>[4x]MTQQITLIKDKILSDNYFTLHNITYDLTRKDGEVIRHKREVYDRGNGATILLYNTKKKTVVLIRQFRVATWVNGNESGQLIE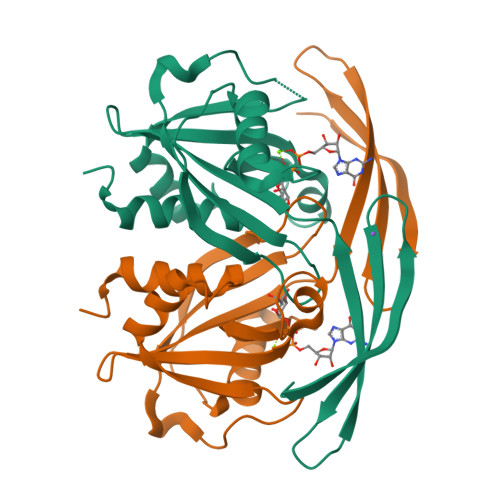SCAGLLDNDEPEVCIRKAAIEETGYEVGEVRKLFELYMSPGGVTELIHFFIAEYSDNQRANAGGGVEDEDIEVLELPFSQALEMIKTGEIRDGKTVLLLNYLQTSHLMD>[4x]AVSKVYARSVYDSRGNPTVEVELTTEKGVFRSIVPSGAATGVHEALEMRDGDKSKWMGKGVLHAVKNVNDVIAPAFVKANIDVKDQKAVDDFLISLDGTANKSKLGANAILGVSLAASRAAAAEKNVPLYKHLADLSKSKTSPYVLPVPFLNVLNGGSHAGGALALQEFMI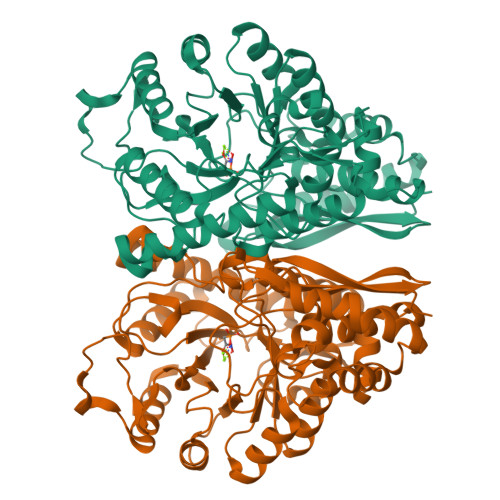APTGAKTFAEALRIGSEVYHNLKSLTKKRYGASAGNVGDEGGVAPNIQTAEEALDLIVDAIKAAGHDGKVKIGLDCASSEFFKDGKYDLDFKNPNSDKSKWLTGPQLADLYHSLMKRYPIVSIEDPFAEDDWEAWSHFFKTAGIQIVADDLTVTNPKRIATAIEKKAADALLLKVNQIGTLSESIKAAQDSFAAGWGVMVSHRSGETEDTFIADLVVGLRTGQIKTGAPARSERLAKLNQLLRIEEELGDNAVFAGENFHHGDKL> MELDDALDELSDSLGQRQPDPDENKPLDDKVKEKIKAEHSEK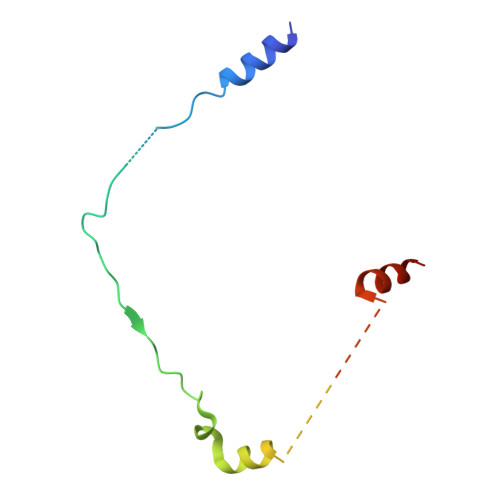LGERDDTIPPEYRHLLDNDGKDKPEKPLTKNTEKPGQDQDPIDALSEDLDSCP>MAANSTRRPIIAFMSDLGTTDDSVAQCKGLMYSICPDVTVVDVCHSMTPWDVEEGARYIVDLPRFFPEGTVFATTTYPATGTTTRSVAV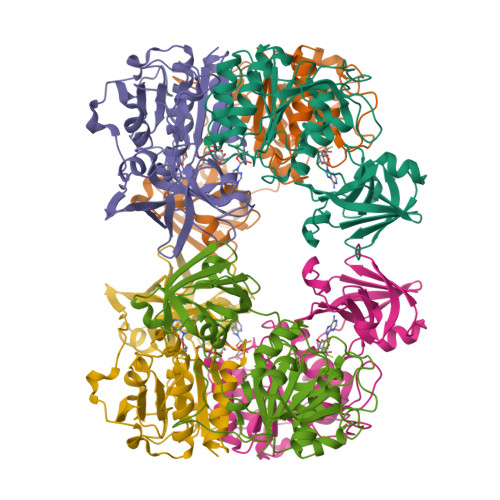RIKQAAKGGARGQWAGSGAGFERAEGSYIYIAPNNGLLTTVLEEHGYLEAYEVTSPKVIPEQPEPTFYSREMVAIPSAHLAAGFPLSEVGRPLEDHEIVRFNRPAVEQDGEALVGVVSAIDHPFGNVWTNIHRTDLEKAGIGYGARLRLTLDGVLPFEAPLTPTFADAGEIGNIAIYLNSRGYLSIARNAASLAYPYHLKEGMSARVEAR[3x]>MVRGIRGAITVEEDTPAAILAATIELLLKMLEANGIQSYEELAAVIFTVTEDLTSAFPAEAARLIGMHRVPLLSAREVPVPGSLPRVIRVLALWNTDTPQDRVRHVYLNEAVRLRPDLESAQLEHHHHHH[12x];>MEEVVLITVPSA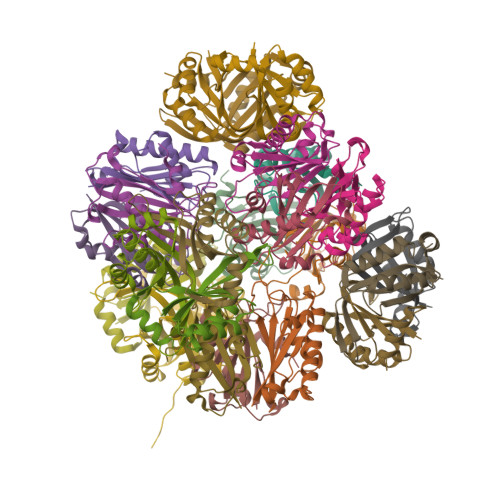LVAVKIAHALVEERLAACVNIVPGLTSIYREEGSVVSDHELLLLVKTTTDAFPKLKERVKELHPYEVPEIVALPIAEGNREYLDWLRENTGLEHHHHHH[12x]> MHHHHHHMIEELGKIDRIIQESVPGKQITLAHVIAAPIEAVYECLGVDHEGAIGVVSLTPNETAIIAADIAGAAANIDICFVDRFTGSVMFSGDI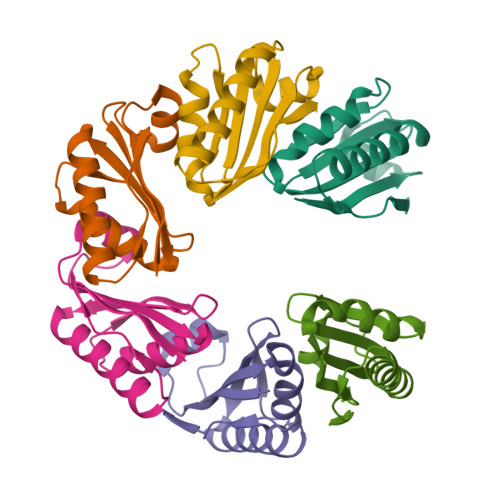QSVETSLEDILEYFKNSLGFSTVPLTKS methyl 2-[2-(3,5-dihydro-2~{H}-pyrazin-4-yl)ethoxy]-5-[(5-ethanoyl-2-ethoxy-phenyl)carbamoyl]benzoate 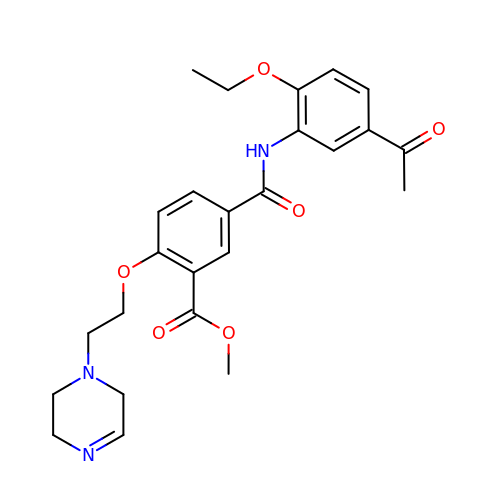| C25 H29 N3 O6 | HFLCQGIXUOKAGP-UHFFFAOYSA-N2-azanyl-7-[(2~{S},3~{R},5~{S})-5-(hydroxymethyl)-3-oxidanyl-pyrrolidin-2-yl]-3,5-dihydropyrrolo[3,2-d]pyrimidin-4-one 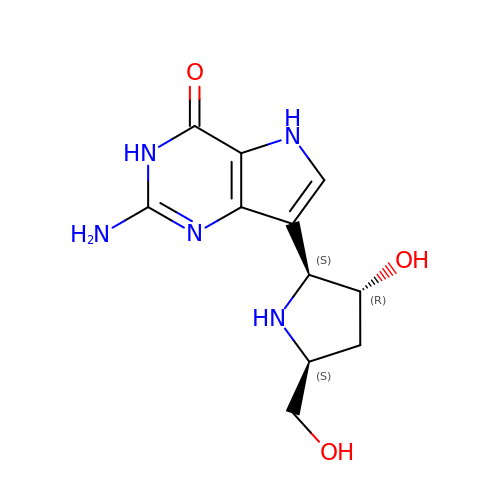| C11 H15 N5 O3 | ZIWDWRULEXWPGT-JHYUDYDFSA-N>HHHHHHTGLDLGAASSFGALAPQGVANAGATVINGDMGTTGTSITGFPPGLITGQLHINDDTSTQAFADSRTAFVAGQALIATVDQAGTATLGGNTFVAGVYKYDSAVGLDGVLTLDGAGDASSVWVFQLATTLVTYASSSIILTNGAKANNVFWIVGYSATLGTYSHLEGNVIANALIAAQTGATINGALLAGSAVTLDSNTVTVQNSASKLVRSAKFFKV[3x]

Here we present new structural data for an IBP identified from a cold-tolerant fungus, Antarctomyces psychrotrophicus (AnpIBP). The structure of AnpIBP consists of a 45-Å-long β-helical fold with a triangular cross section. The main constituents are 6-ladder β-helical loops, which are supported by a long α-helix located along the β-helical axis. The AnpIBP uniquely binds to the water molecules that participate in the primary and secondary prism planes, which were detected as a prism ring in the FIPA experiment.

We examined such water molecules located on the crystal structures of AnpIBP and the S153Y mutants. In crystals of AnpIBP and S153Y, the asymmetric unit contained six molecules and three molecules, respectively. Mutations in S153Y and T156Y on the B-face resulted in a decrease in activity to 17% of the wild-type. All AnpIBP mutants exhibited highly similar CD profiles to the wild-type, suggesting that defective mutations did not affect the overall structure but collapsed a structure needed for ice binding on the B-face. In contrast, the defective mutant S153Y generated a hexagonal bipyramid, as produced by fish IBPs. In FIPA analysis, the illumination of S153Y was observed in six patches at the middle latitude of the ice hemisphere. This result indicates that the S153Y mutant loses the binding affinity to the prism ring, as it occupies the equator. There are at least 13 polygons on the IBS of AnpIBP, which are mainly located around S153 and T156. Such ice-like polygonally arranged water molecules were not identified on the solvent-exposed IBS of a mutant, S153Y, whose TH activity and ice-binding ability were lowered. The illumination area of T156Y was further reduced in comparison with that of the S153Y mutant, suggesting a significant loss of binding ability. These results suggest that Ser153 and Thr156 on the B-face are the residues necessary to bind to the water molecules constructing the prism ring of a single ice crystal hemisphere.>MPMILGYWDIRGLAHAIRLLLE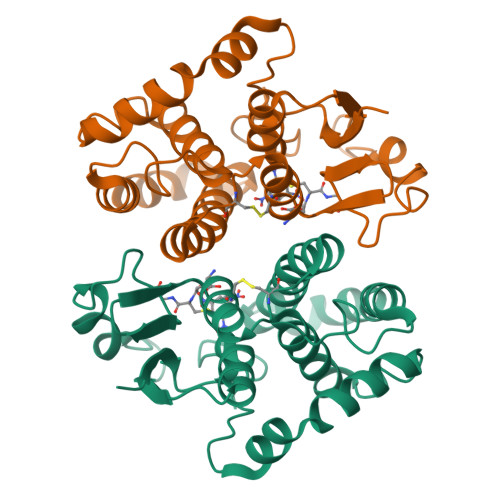YTDSSYEEKKYTMGDAPDYDRSQWLNEKFKLGLDFPNLPYLIDGAHKITQSNAILCYIARKHNLCGETEEEKIRVDILENQTMDNHMQLGMICYNPEFEKLKPKYLEELPEKLKLYSEFLGKRPWFAGNKITFVDFLVYDVLDLHRIFEPKCLDAFPNLKDFISRFEGLEKISAYMKSSRFLPRPVFSKMAVWGNK[6x]>[2x]GMPRPKLKSDDEVLEAATVVLKRCGPIEFTLSGVAKEVGLSRAA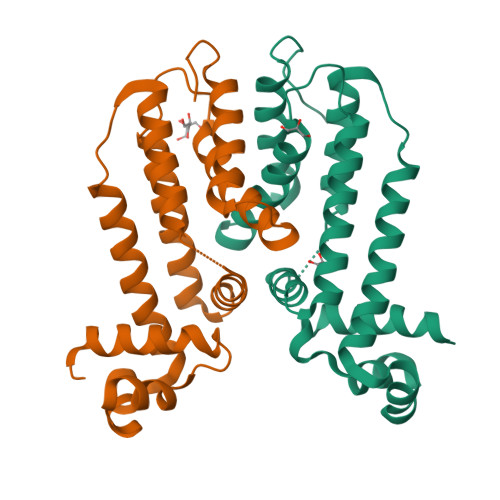LIQRFTNRDTLLVRMMERGVEQVRHYLNAIPIGAGPQGLWEFLQVLVRSMNTRNDFSVNYLISWYELQVPELRTLAIQRNRAVVEGIRKRLPPGAPAAAELLLHSVIAGATMQWAVDPDGELADHVLAQIAAILCLMFPEHDDFQLLQAHA~{N}-(phenylmethyl)pyridine-2-carboxamide 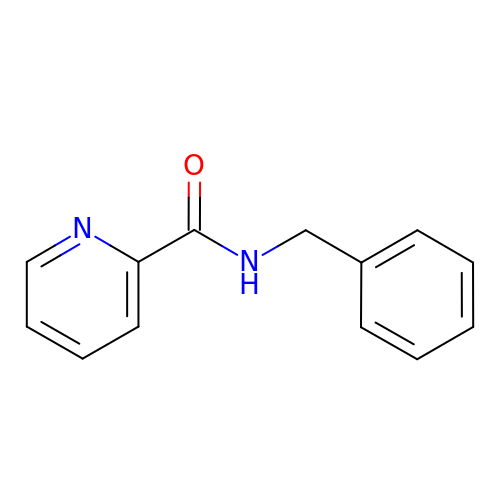| C13 H12 N2 O | NNIFYECULHSHBH-UHFFFAOYSA-N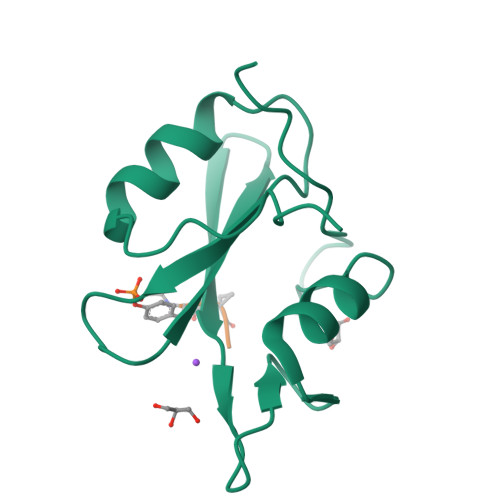> IEMKPHPWFFGKIPRAKAEEMLSKQRHDGAFLIRESESAPGDFSLSVKFGNDVQHFKVLRDGAGKYFLWVVKFNSLNELVDYHRSTSVSRNQQIFLRDIEQVPQQPTYVQAHHHHHH>MKVVDISKINELVKEGATLMIGGFLGVGTPENIIDEIIRHNISNLTVIANDTAFEDRGIGKLVKNKLCKKVIVSHIGTNPETQRQMIEGTLEVELVPQGTLAERIRAAGVGLGGILTPTGVGTVVEKDKKVIEVEGKKYLLELPIHADVALIKAKKADYLGNLVYNLTAENFNPIMALAAKTVIAEVEEIVPTGTLSPNEIKTPGIIVDYIVTGVTR[2x];>[2x]MNPKEKIAIRVAQELKKGQLVNLGIGLPTLVANYIPKDIHVFFQSSNGIIGMGPAPKEGYENSDLTNAGASYITALPGAMTFDSAFSFGIIRGGHLDVTVLGGLQVDEEGHLANWMIPGKMIPGMGGAMDLVTGAKKVIVAMTHTAKGTPKIVKKCTLPLTSIRKVDLIVTELAVIEPTDEGLLLKEISKETTLDEVLKLTEAKLIIADDLKIFA

CtfAB then transfers the CoA from acetoacetyl-CoA to acetate to reform an acetyl-CoA and produce acetoacetate. CtfAB is a member of family 1 CoA transferases. CtfB contains the acetyl-CoA binding site and the PS01724 signature sequence which includes the catalytic glutamate residue (E46) sandwiched between two short antiparallel beta strands on the N-terminal end of an eight-stranded mixed beta sheet. CtfA contains the acetate binding site and the PS01723 signature sequence.

Additional support for the necessity of a carboxylate is that mutation of the catalytic glutamate to serine results in a catalytically inactive enzyme that cannot catalyze either the CoA transferase or hydrolase reaction. The E46S mutant is catalytically inactive. The E46S mutant hydroxyl group is not within hydrogen bond distance of any protein atoms. Instead, a second acetate molecule binds in the space normally occupied by the catalytic glutamate carboxylate, 3.2 Å from the E46S hydroxyl. Acetate molecules were identified in every CtfAB structure in the substrate-binding pocket directly adjacent to catalytic residue E46.>[2x]MSFINYSSREINCKIVYYGPGLCGKTTNLQYIYNKTAAETKGKLISLSTETDRTLFFDFLPLSLGEIRGFKTRFHLYTVPGQVFYD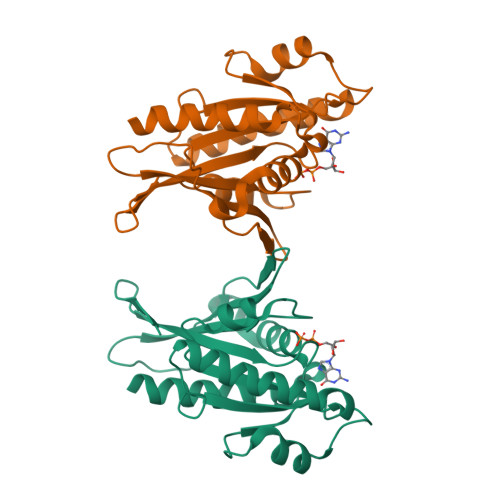ASRKLILKGVDGVVFVADSQIERMEANMESLENLRINLAEQGYDLNKIPYVIQYNKRDLPNAVTVEEMRKALNHRNIPEYQAVAPTGVGVFDTLKAVAKLVLTELKKGG>GPMSDEQTFIAIKPDGVQRGLVGPIISRFENRGFKLAALKLCSPSKEHLEQHYADLSSKPFFPGLVSYMLSGPIVAMVWEGREVVKTGRTILGATNPLASAPGTIRGDFAIDVGRNVCHGSDSVENAKKEIALWFKPEELQK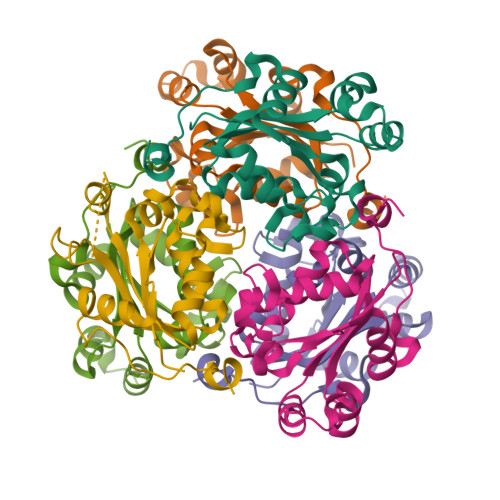YKHSQFDWIYEKA[24x]> CG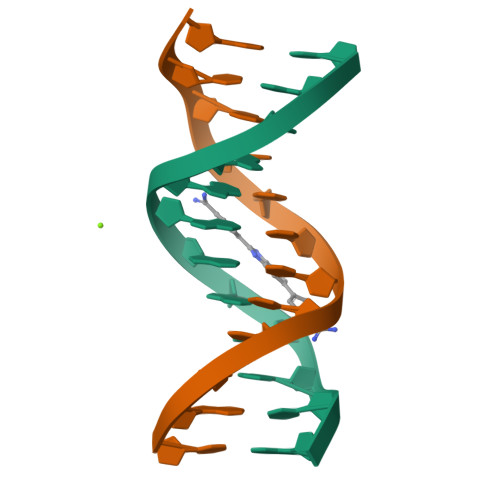CAAAAAAGCG;> CGCTTTTTTGCG> AHYNTEILKSIDNEWRKTQCMPREVAIDVGKEFGVATNTFFKPPCVSVYRCGGCCNSEGLQCMNTSTSYLSKTLFEITVPLSQGPKPVTISFANHTSCRCMSKLHHHHHH;> DYRSPFIASVSDQHGVVY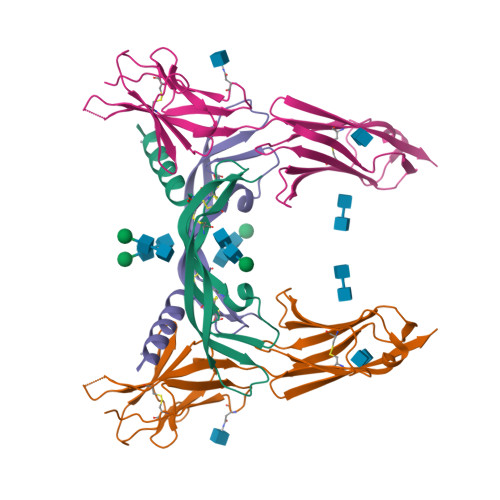ITENKNKTVVIPCLGSISNLNVSLCARYPEKRFVPDGNRISWDSKKGFTIPSYMISYAGMVFCEAKINDESYQSIMYIVVVVGYRIYDVVLSPSHGIELSVGEKLVLNCTARTELNVGIDFNWEYPSSKHQHKKLVNRDLKTQSGSEMKKFLSTLTIDGVTRSDQGLYTCAASSGLMTKKNSTFVRVHEDPIEGR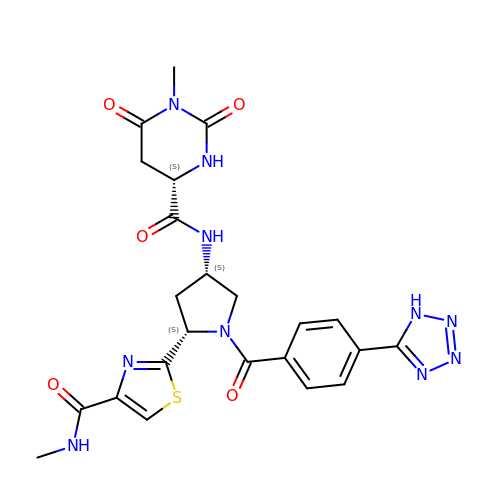(4S)-1-methyl-N-{(3S,5S)-5-[4-(methylcarbamoyl)-1,3-thiazol-2-yl]-1-[4-(1H-tetrazol-5-yl)benzene-1-carbonyl]pyrrolidin-3-yl}-2,6-dioxohexahydropyrimidine-4-carboxamide | C23 H24 N10 O5 S | SYFLGRBSBZONAM-DZKIICNBSA-N> ARLNRESVIDAALELLNETGIDGLTTRKLAQKLGIEQPTLYWHVKNKR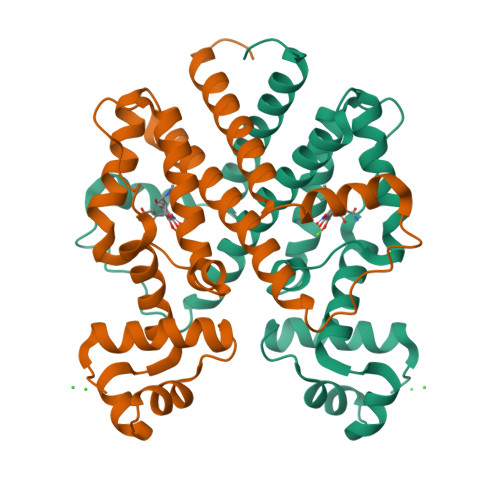ALLDALAVEILARHHDYSLPAAGESWQSFLRNNAMSFRRALLRYRDGAKVHLGTRPDEKQYDTVETQLRFMTENGFSLRDGLYAISAVSHFTLGAVLEQQEHTAALTDRPAAPDENLPPLLREALQIMDSDDGEQAFLHGLESLIRGFEVQLTALLQIV> MERNKLARQIIDTCLEMTRLGLNQGTAGNVSVRYQDGMLITPTGIPYEKLTESHIVFIDGNGKHEEGKLPSSEWRFHMAAYQSRPDANAVVHNHAVHCTAVSILNRSIPAIHFM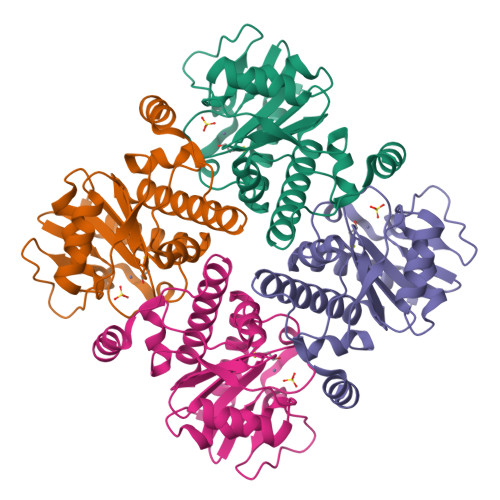IAAAGGNSIPCAPYATFGTRELSEHVALALKNRKATLLQHHGLIACEVNLEKALWLAHEVEVLAQLYLTTLAITDPVPVLSDEEIAVVLEKFKTFGLRIEE>[2x]GSMIPSITAYDALGLKIEFTFERSNTNPSVTVITIQASN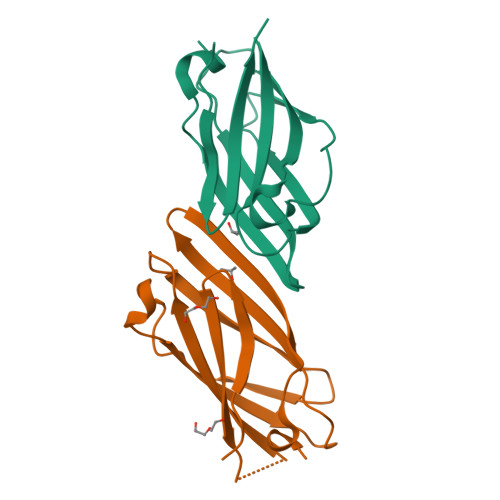STELDMTDFVFQAAVPKTFQLQLLSPSSSVVPAFNTGTITQVIKVLNPQKQQLRMRIKLTFNWNGYKVQSEAEVNNFPPQSWQ>[2x]GMRQAKTDLAEQIFSATDRLMAREGLNQLSMLKLAKEANVAAGTIYLYFKNKDELLEQFAHRVFSMFMATLEKDFDETKPFFEQYRQMWKNIWYFLQEN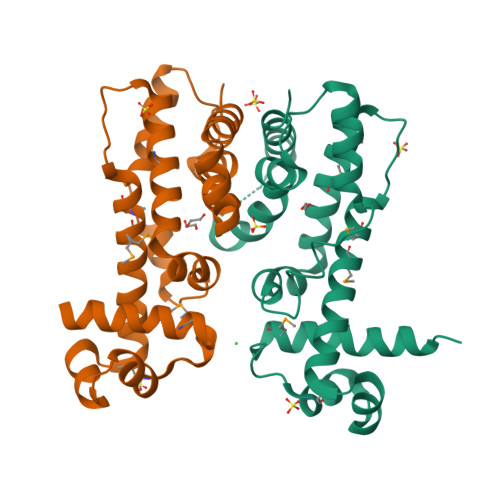PTILSNLKQYESLPNFKDICKNIKNCRWDLFCHQAQKAGLLAELSEDILFLLSLKTAINLASDAKFIDFDLKPEILESVIERSWRAIQK> DD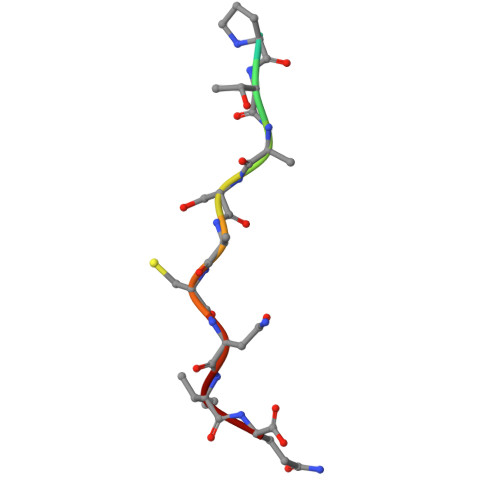PTASACNIQ> GLYLQVGAFANPDAAELLKAKLSGVTAAPVFISSVVRNQQILHRVRLGPIGSADEVSRTQDSIRVANLGQPTLVRPD

However, it is known that the sporulation-related repeat (SPOR) domains (Pfam 05036), ubiquitous in prokaryotes, play a central role in directing proteins to the septum by recognition of the unique septal PG (rather than recognition by other division proteins), which is enriched in denuded glycans, the PG devoid of peptide stems. Of all SPOR-domain-containing proteins, RlpA is the most highly conserved across bacterial species, which underscores its important physiological role in bacteria. It is predicted to have two domains, a catalytic “double-ψ β-barrel” domain (DPBB; Pfam 03330) and a C-terminal SPOR domain. In the present report, we disclose the X-ray structure of the SPOR domain of rare lipoprotein A (RlpA) from P. aeruginosa (SPOR-RlpA).

In order to characterize how the SPOR-RlpA domain interacts with denuded PG, we solved the X-ray structure of the complex with compound 1. Co-crystallization and soaking were both performed in parallel and resulted in two structures for the SPOR-RlpA:1 complex at near-atomic resolution (1.30 and 1.48 Å, respectively). The two structures are identical (rmsd of 0.16 Å for the 77 Cα atoms); the description provided herein is for the 1.30 Å resolution cocrystallization complex. The electron-density for compound 1 bound to the SPOR domain is excellent. The PG-binding site in the SPOR domain is located within the concave face of the β-sheet (the “palm” side in the top depiction of Fig. 4a), presenting a short funnel-like cavity (15 Å long by a width raging from 8–18 Å) in which the tetrasaccharide is ensconced in an extended conformation. The positions of the sugar units have been labeled 1 to 4, corresponding to NAM(1), NAG(2), NAM(3), NAG(4). The largest number of interactions is observed for NAM(1) (eight polar interactions with four atoms in the NAM), and to a lesser extent with NAG(2) (four polar interactions with three atoms in the NAG) and NAM(3) (five polar interactions with four atoms in the NAM). (iv) Several amino acids participate in the stabilization of the tetrasaccharide, but only the side chains of Q270, R302 and R309 are directly involved in the interaction with the glycan chain through polar interactions with oxygen atoms of the carboxylate of the lactyl moiety and the N-acetyls of NAM(1) and NAG(2). It is noteworthy that these residues, together with R311, build a basic patch critical for the binding of the carboxylate and acetyl groups of NAM(1). Most of residues contribute to the stabilization of the glycan chain by the formation of hydrogen bonds with the protein backbone (residues 271, 273, 275, 276, 333, and 335) or by stabilization of the hydrogen-bond network mediated by water molecules.(3S)-N-(9H-xanthen-9-ylmethyl)piperidine-3-carboxamide | C20 H22 N2 O2 | 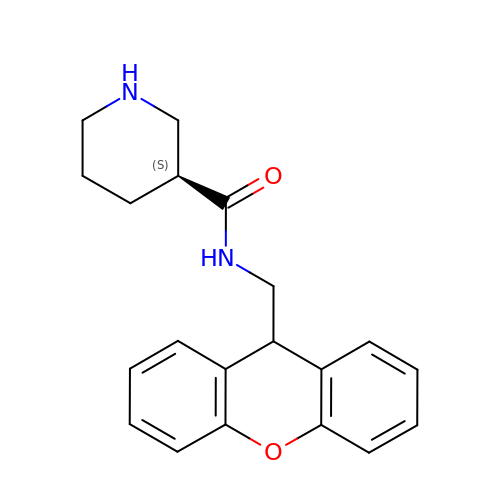WUFJDXQJUMCLAA-AWEZNQCLSA-N4-(2-chlorophenyl)-8-(2-hydroxyethyl)-6-methylpyrrolo[3,4-e]indole-1,3(2H,6H)-dione 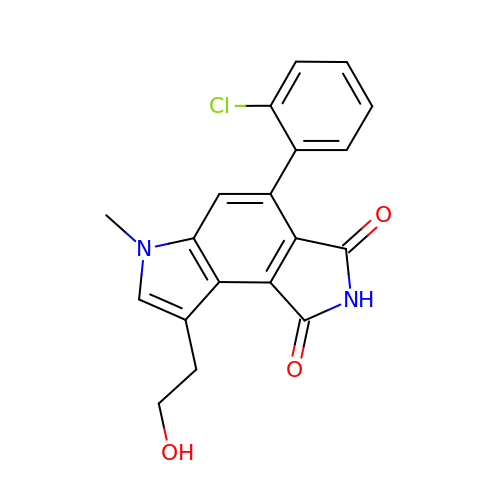| C19 H15 Cl N2 O3 | WHMQZCPGFZBLBG-UHFFFAOYSA-N> MAQARKIPLDLPGTRILNGANWANNSATENLATNSGTLIIFDQSTPGQDADRWLIH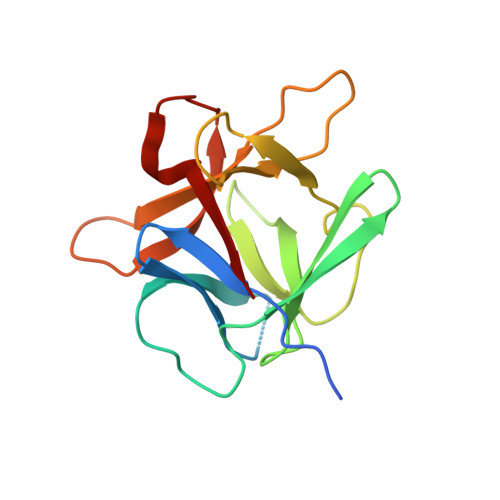NYLDGYKIFNMGSNNWASVSRGNTVLGVSEFDGQTCKWSIEYSGNGEEFWIRVPREGGGGAVWTIKPASSQGPTTVFLDLLKETDPNQRIKFAV>[4x]ADSDVPNDILEEQLYNSVVVADYDSAVEKSKHLYEEKKSEVITNVVNKLIRNNKMNCMEYAYQLWLQGSKDIVRDCFPVEFRLIFAENAIKLMYKRDGLALTLSNDVQGDDGRPAYGDGKDKTSPRVSWKLIALWENNKVYFKILNTERNQYLVLGVGTNWNGDHMAFGVNSVDSFRAQWYLQPAKYDNDVLFYIYNREYSKALTLSRTVEPSGHRMAWGYNGRVIGSPEHYAWGIKAF

The study reports two crystal structures of Bmlp3, a protein belonging to the 30-kDa lipoprotein family found in silkworm hemolymph. Members of the 30-kDa lipoprotein family are the most abundant protein fraction in the hemolymph of silkworm fifth instar larvae. The Bmlp3 molecule consists of a helical N-terminal domain (NTD, residues 1–87) and a β-trefoil C-terminal domain (CTD, residues 88–239). The NTD consists of six helices forming a right-handed superhelix and is classified as a VHS domain.

All Bmlp3 crystals are monoclinic but belong to different space groups, P21 (Bmlp3-p21) and C2 (Bmlp3-c2). The starting model for Bmlp3-p21 was the structure of Bmlp7 and the molecular replacement procedure identified four protein chains in the asymmetric unit. The first important aspect is that each protein molecule traced in the Bmlp3-p21 structure contains all residues of the mature protein; it presents, therefore, the first complete model of a 30-kDa lipoprotein. The electron density was clearly defined for all N-terminal residues, which form a single α-helical turn. The asymmetric unit of Bmlp3-p21 contains four monomeric protein molecules, whereas in the asymmetric unit of Bmlp3-c2 two protein molecules form a dimer. In the Bmlp3-p21 structure, the NTD and CTD fragments are arranged alternately in a head-to-tail fashion, so that residues of the NTD have contacts with residues of the CTD. Although the protein molecules in Bmlp3-p21 are packed more tightly than in Bmlp3-c2 and the solvent content is lower, the results from PISA indicate that in the Bmlp3-p21 structure there are no specific interactions leading to a stable quaternary structure. The crystals of Bmlp3-p21 were obtained with PEG MME 550 as the main precipitant, whereas ammonium sulfate was the precipitant in the Bmlp3-c2 case. pH was also different, 6.5 and 5.5, respectively. In the Bmlp3-p21 structure this cavity is occupied by a fragment of polyethylene glycol (PEG) from the crystallization solution. Through its ether/alcohol character, PEG is a relatively good mimic of a carbohydrate moiety.> S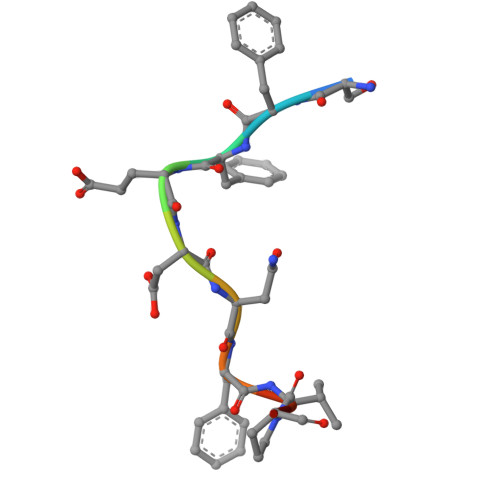FFEDNFVPE> PPTEPLPDGWIMTFHNSGLPVYLHRETRVVTWSRPYFLGTGS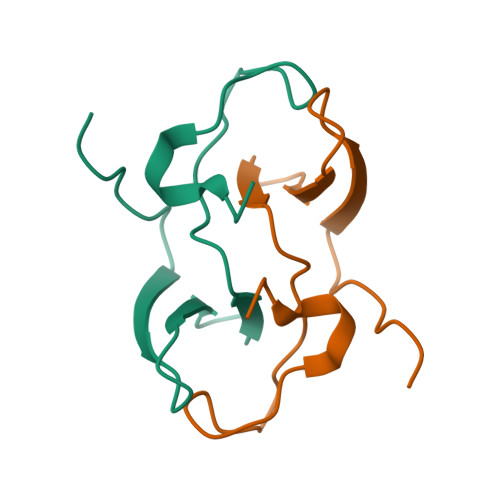IRKHDPPISSIPCL> MNSNRTPSQKVLARQEKIKAVALELFLTKGYQETSLSDIIKLSGGSYSNIYDGFKSKEGLFFEILDDICKKHFHLIYSKTQEIKNGTLKEILTSFGLAFIEIFNQPEAVAFGKIIYSQVYDKDRHLANWIENNQQNFSYNILMGFFKQQNNSYMKKNAEKLAVLFCTMLKEPY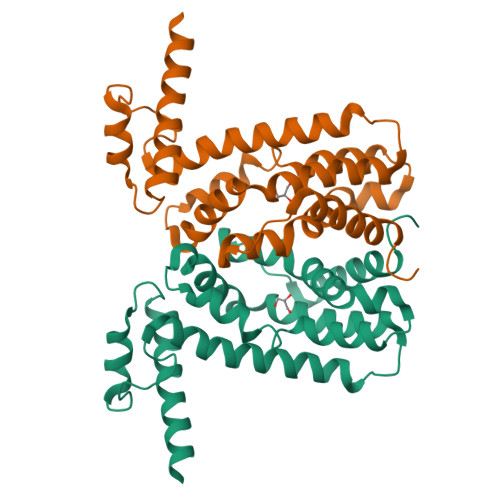HHLNVLINAPLKNKKEQKEHVEFVVNVFLNGINSSKA(2~{R},3~{S},4~{S},5~{S},6~{S})-2-(hydroxymethyl)-6-[(2~{R},3~{S},4~{R},5~{R},6~{R})-2-(hydroxymethyl)-6-[2-[[(2~{R},3~{S},4~{R},5~{R},6~{S})-6-(hydroxymethyl)-5-[(2~{S},3~{R},4~{S},5~{S},6~{R})-6-(hydroxymethyl)-3,4,5-tris(oxidanyl)oxan-2-yl]oxy-3,4-bis(oxidanyl)oxan-2-yl]oxymethyl]-4-[(1~{R},2~{R},4~{S},5'~{R},6~{R},7~{R},8~{R},9~{S},12~{S},13~{R},16~{S})-5',7,9,13-tetramethylspiro[5-oxapentacyclo[10.8.0.0^{2,9}.0^{4,8}.0^{13,18}]icos-18-ene-6,2'-oxane]-16-yl]oxy-butoxy]-4,5-bis(oxidanyl)oxan-3-yl]oxy-oxane-3,4,5-triol 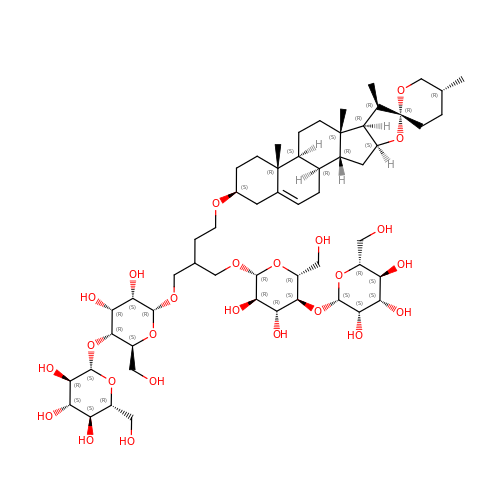| C56 H92 O25 | LKBFXDNKNZXHHW-RFRGGUJUSA-N>MAGDSEQTLQNHQQPNGGEPFLIGVSGGTASGKSSVCAKIVQLLGQNEVDYRQKQVVILSQDSFYRVLTSEQKAKALKGQFNFDHPDAFDNELILKTLKEITEGKTVQIPVYDFVSHSRKEETVTVYPADVVLFEGILAFY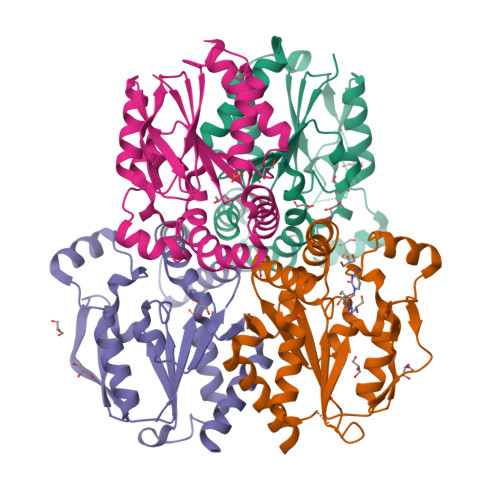SQEVRDLFQMKLFVDTDADTRLSRRVLRDISERGRDLEQILSQYITFVKPAFEEFCLPTKKYADVIIPRGADNLVAINLIVQHIQDILNGGPSKRQTNGCLNGYTPSRK[8x]Next, a β-keto acid cleavage enzyme (BKACE)28,29 converts the non-native substrate MSA with acetyl-CoA into acetoacetate and formyl-CoA. The Claisen-like condensation reaction accepts various β-keto acids that react with acetyl-CoA to form an acyl-CoA ester and acetoacetate. In these assays, BKACE15 from Paracoccus denitrificans performed best. BKACE15 forms a homotetramer where each active site is accommodated in a TIM-barrel fold, and consists of eight β-sheets that are surrounded by eight α-helices.

The four monomers of the tetrameric complex are indicated by different colors. Substrate labeling is shown in yellow for acetyl-CoA (“ACO”) and acetoacetate (“AAE”) and in dark grey for CoA (“COA”) and malonate (“MLI”). Malonate, CoA and the corresponding backbone are shown in dark grey, acetoacetate, acetyl-CoA and the corresponding backbone in yellow, zinc (Zn2+) in metal grey, polar interactions in light grey dashes. As previously reported for the BKACE from Candidatus Cloacamonas acidaminovorans, a close homolog of BKACE15, each active site coordinates a single Zn2+ ion. Earlier studies had proposed R254 as a catalytic base involved in the reaction. However, our structures with bound CoA-ester prompted us to revisit the nature of the catalytic base and suggest a different mechanism for the reaction with MSA, in which E171 acts as the catalytic base (discussed in more detail in Supplementary Note 2). Replacing E171 by leucine abolished BKACE activity, while substitution by a chemically similar but shorter aspartate still showed basal activity (5% of the wild type), supporting the role of E171 in catalysis.

>[4x]MGHHHHHHHHHHSSGHIEGRHGSRMSLNGKVIITCAVTGAIHTPSMSPYLPVSASEITDAAIGAAEAGAAVIHLHARHEGDGSPDQSVEAFNPILGVIKQASDAVLNITTGGAPTMSIAERIQPAQHYRPELASLNMGTMNFGLFPMLNRYESQLKHQWERNYLGNKDIIFRNTFGDVEHVMTTLGAGGTRFEFECYDTSHLYNLKHFYDRGLVKGPLFIQTVFGLMGGIGAHPDDVLHMKRTADRLFGQDYRWSVLGAGRNQLNIAAMSAAMGGHVRVGLEDNLWAGKGRLAETNAQQVRAARQIVEGLGLEVATPAEARELLALKGGDQVNF>[2x]TKH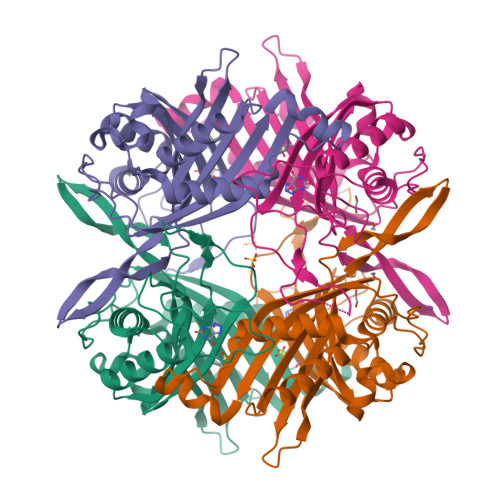KERVMYYGKGDVFAYRTYLKPLTGVRTIPESPFSGRDHILFGVNVKISVGGTKLLTSFTKGDNSLVVATDSMKNFIQKHLASYTGTTIEGFLEYVATSFLKKYSHIEKISLIGEEIPFETTFAVKNGNRAASELVFKKSRNEYATAYLNMVRNEDNTLNITEQQSGLAGLQLIKVSGNSFVGFIRDEYTTLPEDSNRPLFVYLNIKWKYKNTEDSFGTNPENYVAAEQIRDIATSVFHETETLSIQHLIYLIGRRILERFPQLQEVYFESQNHTWDKIVEEIGESEGKVYTEPRPPYGFQCFTVTQEDLPHENILMFSDE> GSMPDYVAKYPVIQTDDERERYKAVFQDQFSEYKELSAEVQAVLRKFDELDAVMSRLPHHSESRQEHERISRIHEEFKKKKNDPTFLEKKERCDYLKNKLSHIKQRIQE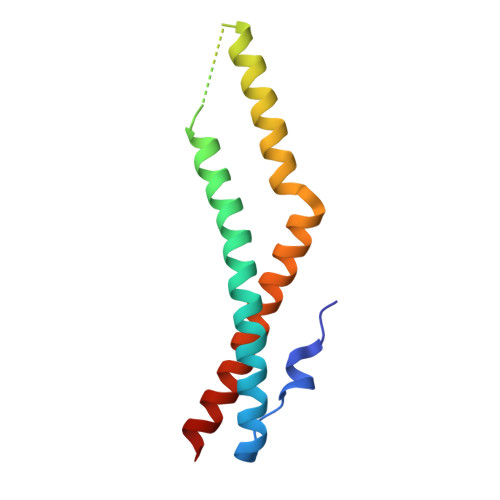YDKVMN>MNTPEHMTAVVQRAVAALNAGDLDGIVALFADDATVEDPVGSEPRSGTAAIREFFANSLKLPLAVELTQE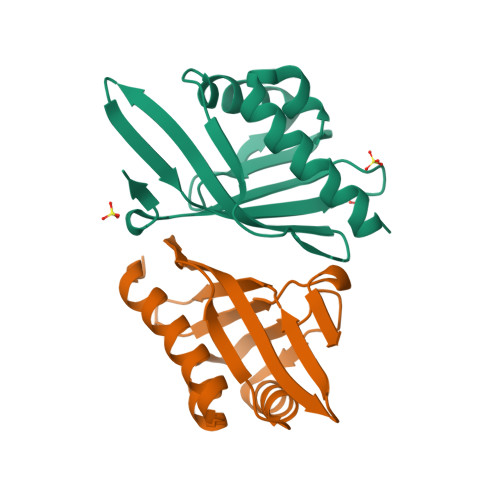VRAVANEAAFAFTVSFEYQGRKTVVAPIAHFRFNGAGKVVSMRALFGEKNIHAGA[4x]~{tert}-butyl 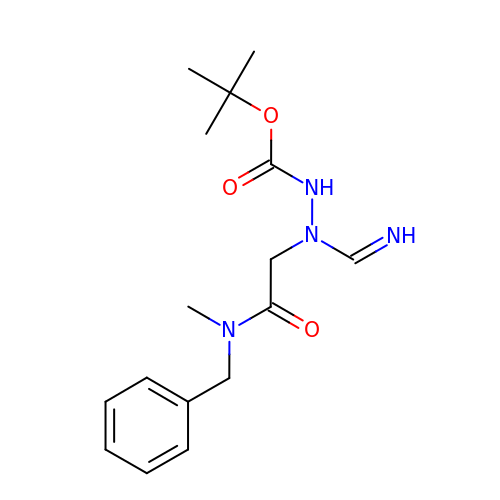~{N}-[iminomethyl-[2-[methyl-(phenylmethyl)amino]-2-oxidanylidene-ethyl]amino]carbamate | C16 H24 N4 O3 | NNHMMRHKBKUPKO-SFQUDFHCSA-N>QSDLLVPKLTASVTDGAVGVTVDAPVSVTAADGVLAAVTMVNDNGRPVAGRLSPDGLRWSTTEQLGYNRRYTLNATALGLGGAATRQLTFQTSSPAHLTMPYVMPGDGEVVGVGEPVAIRFDENIADRGAAEKAIKITTNPPVEGAFYWLNNREVRWRPEHFWKPGTAVDVAVNTYGVDLGEGMFGEDNVQTHFTIGDEVIATADDNTKILTVRVNGEVVKSMPTSMGKDSTPTANGIYIVGSRYKHIIMDSSTYGVPVNSPNGYRTDVDWATQISYSGVFVHSAPWSVGAQGHTNTSHGCLNVSPSNAQWFYDHVKRGDIVEVVNTVGGTLPGIDGLGDWNIPWDQWRAGNAKA[2x]

The L,D-transpeptidase LdtMt2 of Mycobacterium tuberculosis, which is a target for TB treatment, is amenable to covalent inhibition via reaction with its catalytic cysteine. We report αβ,α′β′-diepoxyketones (DEKs) as a new type of mechanism-based inhibitors of nucleophilic cysteine enzymes. Studies with the l,d-transpeptidase LdtMt2 from Mycobacterium tuberculosis and the main protease from SARS-CoV-2 (Mpro) reveal that following epoxide ring opening by a nucleophilic cysteine, further reactions can occur, leading to irreversible alkylation. Here, we describe the identification of the small molecule trans,trans αβ,α′β′-diepoxyketone (DEK) 1, and the potency and mechanism of 1 and related DEKs 4–12 for LdtMt2 and SARS-CoV-2 Mpro inhibition; the results reveal DEKs as a mechanistically interesting class of electrophile.

DEK 1 exhibited potent inhibition of LdtMt2, with a pIC50 of 7.2 ± 0.1, with 30 min pre-incubation. The results reveal that 1 covalently reacts with LdtMt2, giving an initial adduct with a +267 Da mass shift relative to unmodified LdtMt2 (ESI†), corresponding to addition of one molecule of 1 to LdtMt2, which has a single cysteine (Cys354). This adduct was transient, converting within 2 h into one with a mass shift of +160 Da relative to unmodified LdtMt2, provisionally assigned as 3. We proposed the reaction involves nucleophilic attack of Cys354 on the carbonyl-group adjacent carbon of one of the symmetrical epoxides, with ring opening to form 2, followed by retro-aldol fragmentation, releasing benzaldehyde. As reported, LdtMt2 crystallised with two molecules (chains A and B) in the asymmetric unit. While this structure manifested clear additional electron density at the chain A active site, only partial density was observed at that of chain B, thus inhibitor modelling was only performed in chain A. The additional electron density in chain A supports the proposed structure of adduct 3. The carbonyl of 3 projects into the proposed oxyanion hole, formed by the backbone NH groups of His352, Gly353 and Cys354 (distances of 3.0 Å, 3.4 Å and 3.2 Å, respectively). Extensive hydrophobic interactions of 3 with active site residues Tyr318, His352, Trp340, Thr320, and Met303 were observed. To investigate whether the DEKs react selectively with Cys-354 of LdtMt2, we performed protein-observed SPE-MS assays with LdtMt2 that had been preincubated with ebselen, which is known to selectively and irreversibly react with Cys354.16 When 1 and 4–10 were combined with the LdtMt2-ebselen complex, no reaction was observed, evidencing that inhibition arises from at least partially, selective reaction with Cys354 (ESI†). The combined results of the reaction of DEKs with GSH, cysteine, LdtMt2 and SARS-CoV-2 Mpro, imply a conserved reaction mechanism, involving epoxide opening followed by retro-aldol reaction.> EISLNGYGRFGLQYVEDRGVGLEDTIISSRLRINIVGTTETDQGVTFGAK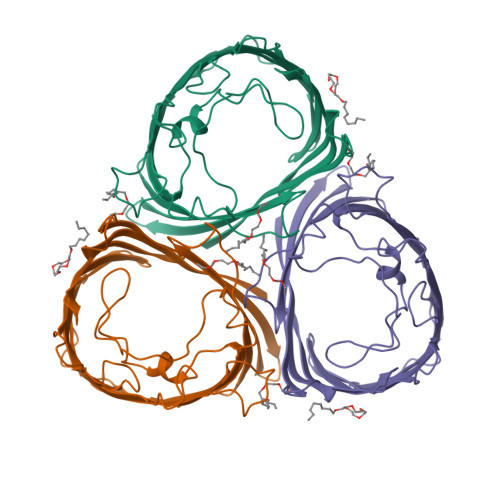LRMQWDDGDAFAGTAGNAAQFWTSYNGVTVSVGNVDTAFDSVALTYDSEMGYEASSFGDAQSSFFAYNSKYDASGALDNYNGIAVTYSISGVNLYLSYVDPDQTVDSSLVTEEFGIAADWSNDMISLAAAYTTDAGGIVDNDIAFVGAAYKFNDAGTVGLNWYDNGLSTAGDQVTLYGNYAFGATTVRAYVSDIDRAGADTAYGIGADYQFAEGVKVSGSVQSGFANETVADVGVRFDF>MHSGIDIRVARPEDAEEIQIIYAPIVLNTAISFEEAVPSVEQMRERISTTLQTYPYLVAVREGRVVGYAYASQHRARAAYRWAVDVTVYVAEGQRRSGIARQLYDVLLPVLKRLGYRSAYAG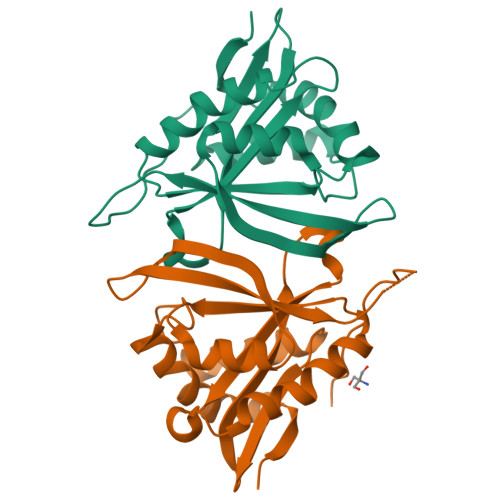IALPNEGSVGLHERLGFQHIGTFPQVGFKLDAWHDVGYWRFDFGDEGLHPEAPLGFLSQIPLGPEQKLISEEDLNSAVDHHHHHH[2x]> MAQTAHQNRYQGGLCYAQCNELFSFWNPSIQQCWKGCDFGVGRVNDPEGR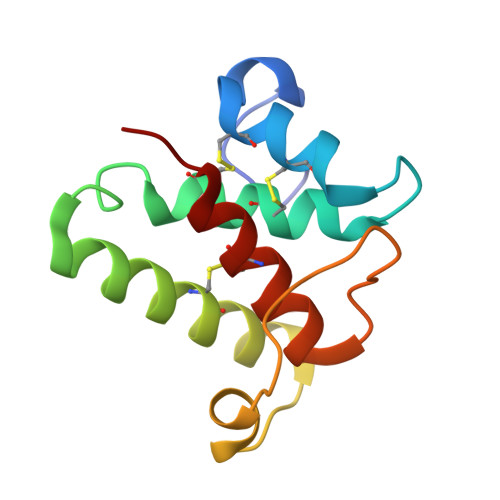IEAQQMCKRWAAELYWTYKGELDTIKDLRVHADMYPTTPQNVYRACLAGVRRQKF>HHHHHHMDAATTRVGLTDLTFRLLRESFADAVSWVAKNLPARPAVPVLSGVLLTGSDNGLTISGFDYEVSAEAQVGAEIVSPGSVLVSGRLLSDITRALPNKPVDVHVEGNRVALTCGNARFSLPTMPVEDYPTLPTLPEETGLLPAEL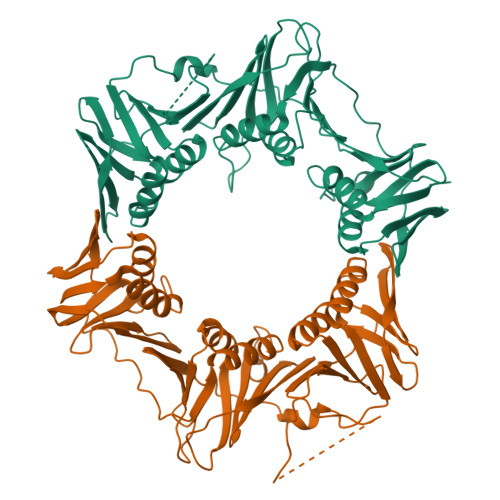FAEAISQVAIAAGRDDTLPMLTGIRVEILGETVVLAATDRFRLAVRELKWSASSPDIEAAVLVPAKTLAEAAKAGIGGSDVRLSLGTGPGVGKDGLLGISGNGKRSTTRLLDAEFPKFRQLLPTEHTAVATMDVAELIEAIKLVALVADRGAQVRMEFADGSVRLSAGADDVGRAEEDLVVDYAGEPLTIAFNPTYLTDGLSSLRSERVSFGFTTAGKPALLRPVSGDDRPVAGLNGNGPFPAVSTDYVYLLMPVRLPG[6x]> GHMNGDQNSDVYAQEKQDFVQHFSQIVRVLTEDEMGHPEI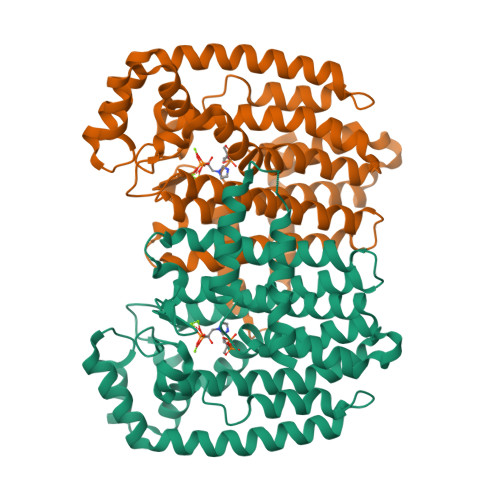GDAIARLKEVLEYNAIGGKYNRGLTVVVAFRELVEPRKQDADSLQRAWTVGWCVELLQAFFLVADDIMDSSLTRRGQICWYQKPGVGLDAINDANLLEACIYRLLKLYCREQPYYLNLIELFLQSSYQTEIGQTLDLLTAPQGNVDLVRFTEKRYKSIVKYKTAFYSFYLPIAAAMYMAGIDGEKEHANAKKILLEMGEFFQIQDDYLDLFGDPSVTGKIGTDIQDNKCSWLVVQCLQRATPEQYQILKENYGQKEAEKVARVKALYEELDLPAVFLQYEEDSYSHIMALIEQYAAPLPPAVFLGLARKIYKRRK SecA is a cytosolic ATPase composed of multiple domains that undergo a series of conformational changes associated with the domain movement during the cycles of ATP binding and hydrolysis in the sequential translocation of the target protein through the SecY channel. C. difficile SecA2 (CDSecA2) is involved in the export of the cell wall proteins (Cwps) that compose the outermost layer of C. difficile, the S-layer. We therefore determined two crystal structures of the CDSecA2 protein (apo and in complex with adenosine-5′-(γ-thio)-triphosphate (ATP-γ-S)). Crystal structures show that CDSecA2 has a fold similar to its homologues, with multidomain organization consisting of NBD1, NBD2, PPXD, HSD and HWD, but lacks CTT.

The crystal of the CDSecA2 and ATP-γ-S complex diffracted considerably worse than the apo structure with a notable anisotropic component. Correspondingly, its structure was less well resolved. Nevertheless, the electron density map for the ATP-γ-S ligand unambiguously positioned it in the active site. The structures of apo CDSecA2 and CDSecA2-ATP-γ-S complex were very similar as they aligned with RMSD 0.85 Å. Binding of ATP-γ-S did not lead to any considerable conformational change such as opening of the PPXD. Crystal packing of CDSecA2 requires contacts between PPXD of one and NBD1 and NBD2 of the adjacent SecA2 molecule, therefore larger conformational changes of PPXD would disrupt the crystal lattice. As evident from the CDSecA2-ATP-γ-S complex structure, the highly conserved residues involved in ATP binding and hydrolysis were positioned within Walker motifs A and B at the interface of NBD1 and NBD2, and are present in all SecA homologues, including CDSecA1 and CDSecA2. As in another SecA the opposite side of the gamma phosphate moiety of ATP-γ-S contains the conserved lysine (K106) in Walker motif A in both SecA1 and SecA2 in C. difficile, and the mutation of this lysine is lethal, suggesting its essential role of both systems. From the CDSecA2 structure with the bound nucleotide and residue conservation in structural alignments, we thought that the requirements for ATP binding and hydrolysis were likely similar to those of other SecA ATPases. With respect to the PPXD position and the extent of interactions between one SecA2 molecule and crystallographic symmetry-related molecules, apo and ATP-γ-S-bound CDSecA2 crystallized as a closed monomer.

> MSVIDSILDKADEQEIKKLNVIVDKIDALEDSMKNLSYEELKDMTAIFKNRLKKGETLDDILPEAFAVVREVSKRKLGMRQYRVQLIGGIVIHQGKIAEMKTGEGKTLVEVAPVYLNALTGKGVHVITVNDYLAERDKELMSPVYESLGMTVGVIISNQDPNIRKQQYKCDITYGTNSEFGFDYLRDNMVPDLSHKVQRELNFAIVDEVDSILIDEARTPLIIAGDGDEDLKLYELANSFVKTVKEEDFELDRKDKTIALTASGISKAESFFGITNLTDIKNIELYHHINQALRGHKLMEKDVDYVISNGEVMIVDEFTGRVMDGRRYTDGLHQAIEAKEGVEIKNESKTMATVTYQNFFRLYEKLSGMTGTAKTEEGEFESIYKLNVVQIPTNRPVIRADLHDKVFKTEEEKYSAVVEEIIRIHKTRQPILVGTVSVEKSEKLSKMLKKQGIKHQVLNAKQHDKEAEIISKAGKLDAITIATNMAGRGTDISLGAGDKEEEQEVKDLGGLYVIGTERHESRRIDNQLRGRSGRQGDPGTSRFFVSLEDDVIKLYGGKTIEKLMKRTSSNENTAIESKALTRAIERAQKGVEGKNFEIRKNVLKYDDTINEQRKVIYNERNKVLNDEDIQEDIQKMVKDIIQEAGETYLIGRKRDYYGYFKHLYSTFMPADTLLIPGVDKKSVQEIIDSTYEISKRVYDLKKMMLGIDKVAELEKTVLLKVVDQYWIDHIDAMEQLKQYIGLKSYAQKDPFKEYALEGYDMFEALNKNIREATVQYLYKFN> GSHMFQCNVPLGMESGRIANEQISASSTYSDGRWTPQQSRLHGDDNGWTPNLDSNKEYLQVDLRFLTMLTAIATQGAISRETQNGYYVKSYKLEVSTNGEDWMVYRHGKNHKVFQANNDATEVVLNKLHAPLLTRFVRIRPQTWHSGIALRLELFGCRVTDAPCSNMLGMLSGLIADSQISASSTQEYLWSPSAARLVSSRSGWFPRIPQAQPGEEWLQVDLGTPKTVKGVIIQGARGGDSITAVEARAFVRKFKVSYSLNGKDWEYIQDPRTQQPKLFEGNMHYDTPDIRRFDPIPAQYVRVYPER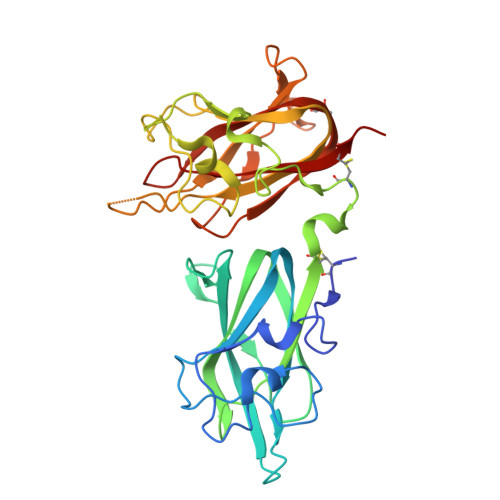WSPAGIGMRLEVLGCDWT> MIYQPDENRYHTMEYRRCGRSGVKLPAISLGLWHNFGDTTRVENSRALLQRAFDLGITHFDLANNYGPPPGSAECNFGRILQEDFLPWRDELIISTKAGYTMWDGPYGDWGSRKY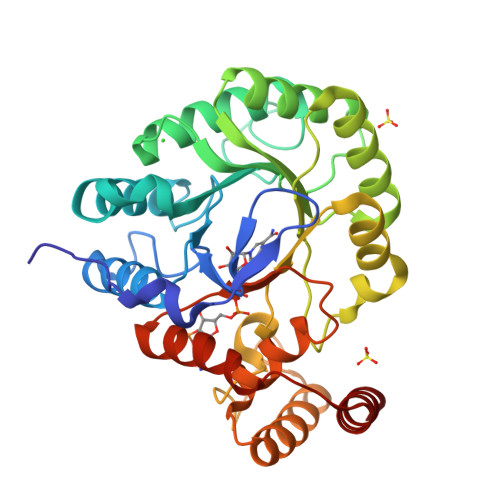LIASLDQSLKRMGLEYVDIFYHHRPDPETPLKETMKALDHLVRHGKALYVGISNYPADLARQAIDILEDLGTPCLIHQPKYSLFERWVEDGLLALLQEKGVGSIAFSPLAGGQLTDRYLNGIPEDSRAASGSRFLKPEQITADKLEKVRRLNELAARRGQKLSQMALAWVLRNDNVTSVLIGASKPSQIEDAVGMLANRRFSAAECAEIDAILEGRF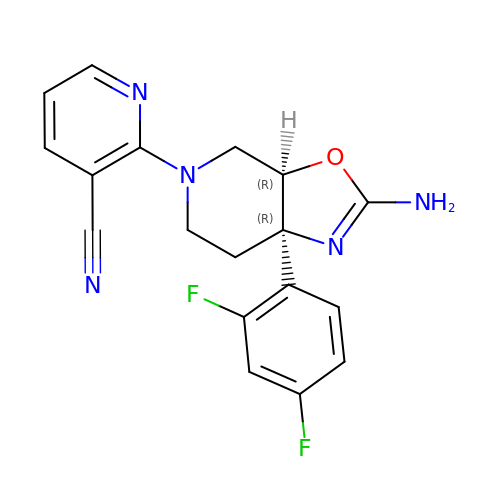2-[(3aR,7aR)-2-amino-7a-(2,4-difluorophenyl)-3a,6,7,7a-tetrahydro[1,3]oxazolo[5,4-c]pyridin-5(4H)-yl]pyridine-3-carbonitrile | C18 H15 F2 N5 O | RDCJBIHDYIOWEV-CRAIPNDOSA-N>[4x]SGGSMLYVSNLPVGTSSSAIHALFSAYGNVKDIWMLSPDNSAIVSY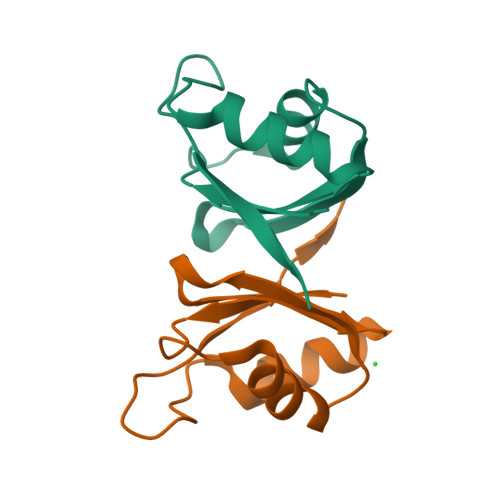ESLSSAIVARDALHNRPVFENHGPVQVMLAKPSSNYE>[2x]SLFELGKMILQE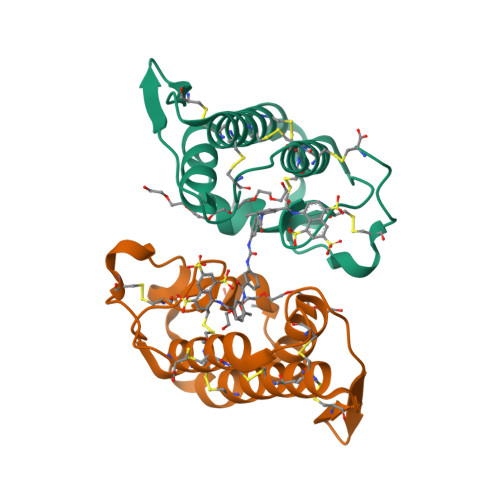TGKNPAKSYGAYGCNCGVLGRGKPKDATDRCCYVHKCCYKKLTGCNPKKDRYSYSWKDKTIVCGENNSCLKELCECDKAVAICLRENLNTYNKKYRYYLKPLCKKADAC> MSEIGTGFPFDPHYVEVLGERMHYVDVGPRDGTPVLFLHGNPTSSYLWRNIIPHVAPSHRCIAPDLIGMGKSDKPDLDYFFDDHVRYLDAFIEALGLEEVVLVIHDWGSALGFHWAKRNPERVKGIACMEFIRPIPTWDEWPEFARELFQAFRTADVGRELIIDQNAFIEQVLPKGVVRPLTEVEMDHYREPFLKPVDREPLWRFPNELPIAGEPANIVALVEA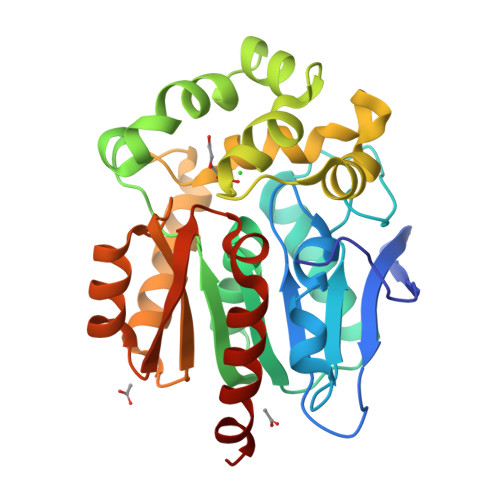YMNWLHQSPVPKLLFWGTPGVLIPPAEAARLAESLPNCKTVDIGPGLHYLQEDNPDLIGSEIARWLPALHHHHHH> RSTLVHWFRKGLRLHDNPALSHIFTAANAAPGRYFVRPIFILDPGILDWMQVGANRWRFLQQTLEDLDNQLRKLNSRLFVVRGKPAEVFPRIFKSWRVEMLTFETDIEPYSVTRDAAVQKLAKAEGVRVETHCSHTIYNPELVIAKNLGKAPITYQKFLGIVEQLKVPKVLGVPEKLKNMPTPPKDEVEQKDSAAYDCPTMKQLVKRPEELGPNKFPGGETEALRRMEESLKDEIWVARFEKPNTAPNSLEPSTTVLSPYLKFGCLSARLFNQKLKEIIKRQPKHSQPPVSLIGQLMWREFYYTVAAAEPNFDRMLGNVYCMQIPWQEHPDHLEAWTHGRTGYPFIDAIMRQLRQEGWIHHLARHAVACFLTRGDLWISWEEGQRVFEQLLLDQDWALNAGNWMWLSASAFFHQYFRVYSPVAFGKKTDPQGHYIRKYVPELSKYPAGCIYEPWKASLVDQRAYGCVLGTDYPHRIVKHEVVHKENIKRMGAAYKVNREV

Here, using femtosecond X-ray crystallography, we report the structural changes that take place while electrons transfer along a chain of four conserved tryptophans in the Drosophila melanogaster (6-4) photolyase. A paradigm for electron-transfer reactions in proteins occurs in photolyases/cryptochromes, where a flavin adenine dinucleotide (FAD) cofactor is photoreduced and electrons are donated through a chain of conserved tryptophan residues. Photolyases repair DNA lesions using light as energy source. In both photolyases and cryptochromes, the photoexcited FAD extracts an electron from the nearby tryptophan, Trp407 (numbered for the Drosophila melanogaster (6-4) photolyase), within 1 ps, initiating a cascade of electron-transfer reactions along Trp384, Trp330 and Trp381.

We recorded time-dependent crystallographic data from microcrystals of Dm(6-4) photolyase dispersed in a cellulose matrix. Next, we turn our attention to the conserved salt bridge between Asp397 and Arg368, which is located on the opposing side of the FAD compared to Asn403. The sulfur atom of Met408 is located only 4.1 Å from the side chain of Trp384. Met408 seems ideal for this because it is located next to the second tryptophan, which does not have many water molecules close by, and methionines can be reversibly oxidized.>[12x]GPLGSMIVFVRFNSSYGFPVEVDSDTSIFQLKEVVAKRQGVP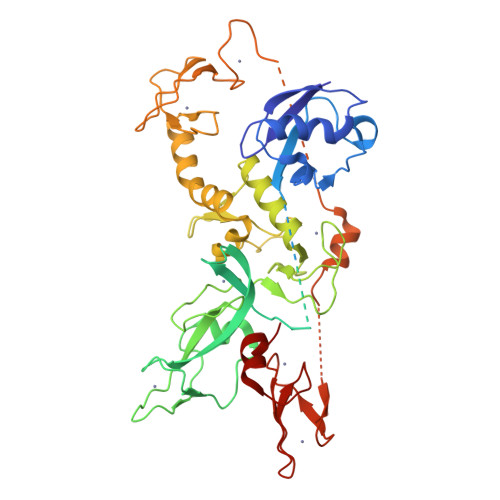ADQLRVIFAGKELQNHLTVQNCDLEQQSIVHIVQRPQRKSHETNASGGDKPQSTPEGSIWEPRSLTRVDLSSHILPADSVGLAVILDTDSKSDSEAARGPAAKPTYHSFFVYCKGPCHKVQPGKLRVQCGTCRQATLTLAQGPSCWDDVLIPNRMSGECQSPDCPGTRAEFFFKCGAHPTSDKDTSVALNLITNNSRSIPCIACTDVRNPVLVFQCNHRHVICLDCFHLYCVTRLNDRQFVHDAQLGYSLPCVAGCPNSLIKELHHFRILGEEQYNRYQQYGAEECVLQMGGVLCPRPGCGAGLLPEQGQRKVTCEGGNGLGCGFVFCRDCKEAYHEGECDSMFEASGATSQAYRVDQRAAEQARWEEASKETIKKTTKPCPRCNVPIEKNGGCMHMKCPQPQCKLEWCWNCGCEWNRACMGDHWFDV>MNAPPALLRSVLFAPGNRADLIAKLPRSAPDAVVIDLEDAVPGTAEAKAAARPVAHDAARDLIAAAPHLAVFVRVNALHSPYFEDDLSVLTPELSGVVVPKLEMGAEARQVAQMLQERSLPLPILAGLETGAGVWNAREIMEVPEVAWAYFGAEDYTTDLGGKRTPGGLEV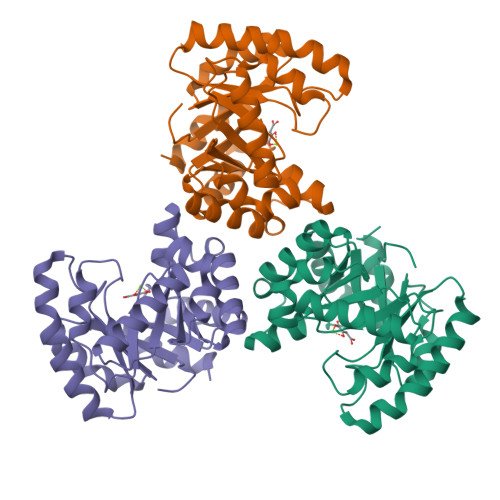LYARSQVALAARLTGVAALDIVVTALNDPETFRADAEQGRALGYSGKLCIHPAQVALAHEYFGPTEADRARARALLDAAAAAAQRGHGAFSFEGQMVDEPMLAKARTLLSHEA[3x]>[2x]MTVEPFRNEPIETFQTEEARRAMREALRRVREEFGR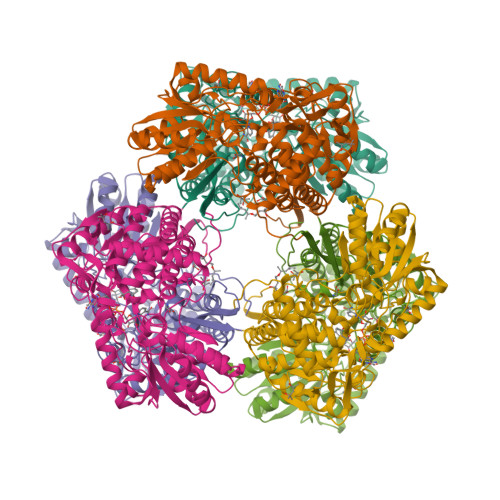HYPLYIGGEWVDTKERMVSLNPSAPSEVVGTTAKAGKAEAEAALEAAWKAFKTWKDWPQEDRSRLLLKAAALMRRRKRELEATLVYEVGKNWVEASADVAEAIDFIEYYARAALRYRYPAVEVVPYPGEDNESFYVPLGAGVVIAPWNFPVAIFTGMIVGPVAVGNTVIAKPAEDAVVVGAKVFEIFHEAGFPPGVVNFLPGVGEEVGAYLVEHPRIRFINFTGSLEVGLKIYEAAGRLAPGQTWFKRAYVETGGKDAIIVDETADFDLAAEGVVVSAYGFQGQKCSAASRLILTQGAYEPVLERVLKRAERLSVGPAEENPDLGPVVSAEQERKVLSYIEIGKNEGQLVLGGKRLEGEGYFIAPTVFTEVPPKARIAQEEIFGPVLSVIRVKDFAEALEVANDTPYGLTGGVYSRKREHLEWARREFHVGNLYFNRKITGALVGVQPFGGFKLSGTNAKTGALDYLRLFLEMKAVAERF>[2x]MNILLVSQCEKRALSETRRILDQFAERRGERTWQTPITQAGLDTLRRLLKKSARRNTAVACHWIRGRDHSELLWIVGDASRFNAQGAVPTNRTCRDILRKEDENDWHSAEDIRLLTVMAALFHDIGKASQAFQAKLRNRGKPMADAYRHEWVSLRLFEAFVGPGSSDEDWLRRLADKRETGDAWLSQLARDDRQSAPPGPFQKSRLPPLAQAVGWLIVSHHRLPNGDHRGSASLARLPAPIQSQWCGARDADAKEKAACWQFPHGLPFASAHWRARTALCAQSMLERPGLLARGPALLHDSYVMHVSRLILMLADHHYSSLPADSRLGDPNFPLHANTDRDSGKLKQRLDEHLLGVALHSRKLAGTLPRLERQLPRLARHKGFTRRVEQPRFRWQDKAYDCAMACREQAMEHGFFGLNLASTGCGKTLANGRILYALADPQRGARFSIALGLRSLTLQTGQAYRERLGLGDDDLAILVGGSAARELFEKQQERLERSGSESAQELLAENSHVHFAGTLEDGPLREWLGRNSAGNRLLQAPILACTIDHLMPASESLRGGHQIAPLLRLMTSDLVLDEVDDFDIDDLPALSRLVHWAGLFGSRVLLSSATLPPALVQGLFEAYRSGREIFQRHRGAPGRATEIRCAWFDEFSSQSSAHGAVTSFSEAHATFVAQRLAKLEQL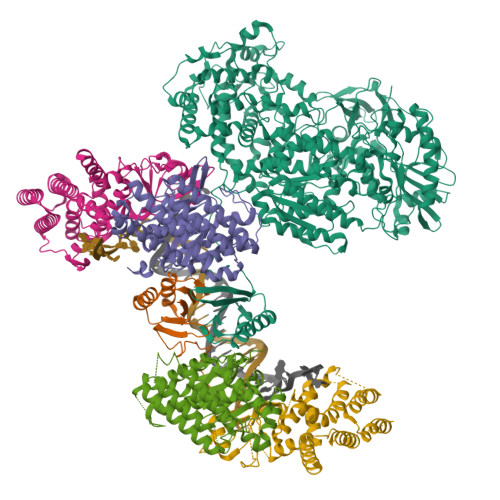PPRRQAQLCTVHAAGEARPALCRELAGQMNTWMADLHRCHHTEHQGRRISFGLLRLANIEPLIELAQAILAQGAPEGLHVHLCVYHSRHPLLVRSAIERQLDELLKRSDDDAAALFARPTLAKALQASTERDHLFVVLASPVAEVGRDHDYDWAIVEPSSMRSIIQLAGRIRRHRSGFSGEANLYLLSRNIRSLEGQNPAFQRPGFETPDFPLDSHDLHDLLDPALLARIDASPRIVEPFPLFPRSRLVDLEHRRLRALMLADDPPSSLLGVPLWWQTPASLSGALQTSQPFRAGAKERCYALLPDEDDEERLHFSRYEEGTWSNQDNLLRNLDLTYGPRIQTWGTVNYREELVAMAGREDLDLRQCAMRYGEVRLRENTQGWSYHPYLGFKKYN;>[4x]MDDISPSELKTILHSKRANLYYLQHCRVLVNGGRVEYVTDEGRHSHYWNIPIANTTSLLLGTGTSITQAAMRELARAGVLVGFCGGGGTPLFSANEVDVEVSWLTPQSEYRPTEYLQRWVGFWFDEEKRLVAARHFQRARLERIRHSWLEDRVLRDAGFAVDATALAVAVEDSARALEQAPNHEHLLTEEARLSKRLFKLAAQATRYGEFVRAKRGSGGDPANRFLDHGNYLAYGLAATATWVLGIPHGLAVLHGKTRRGGLVFDVADLIKDSLILPQAFLSAMRGDEEQDFRQACLDNLSRAQALDFMIDTLKDVAQRSTVSA>MEEKRLSAKKGLPPGTLVYTGKYREDFEIEVMNYSIEEFREFKTTDVESVLPFRDSSTPTWINITGIHRTDVVQRVGEFFGIHPLVLEDILNVHQRPKVEFFENYVFIVLKMFTYDKNLHELESEQVSLILTKNCVLMFQEKIGDVFDPVRERIRYNRGIIRKKRADYLLYSLIDALVDDYFVLLEKIDDEIDVLEEEVLERPEKETVQRTHQLKRNLVELRKTIWPLREVLSSLYRDVPPLIEKETVPYFRDVYDHTIQIADTVETFRDIVSGLLDVYLSSVSNKTNEVMKVLTIIATIFMPLTFIAGIYGMNFEYMPELRWKWGYPVVLAVMGVIAVIMVVYFKKKKWL[10x]

Mg2+ and Co2+ are essential ions for all organisms. In conclusion, CorA transports its substrate in a partially hydrated form.

was of sufficient quality to assign most of the side chains. partially hydrated state (distance of ~4 Å), similar to what was seen in MjCorA and in another recent study on TmCorA. The major differences between the loops of TmCorA and MjCorA are after the YGMNF motif. A similar kink was also observed in the MjCorA structure. hydrophobic pore is completely closed to ions with radii of 4.5 Å or smaller. co-ordination in the metal-binding sites, M1 and M2, as observed in the closed conformation. When the intracellular Co2+ concentration is increased, it will bind to the M2 site.> KQTA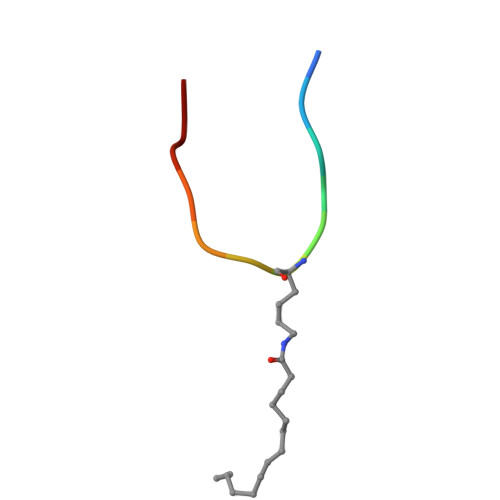RXSTGGWW> XUGCUGGCUAAGGGCCGAAAGX;> CUAUGCCUGCUG

The TNA backbone is composed of phosphodiester-linked 3′→2′ α-l-threofuranose sugars and, therefore, has one fewer atom in its repeating unit than RNA. Critically, TNA can form stable Watson−Crick duplexes with itself, DNA and RNA, such that the exchange of genetic information between these polymers appears feasible. Here, we examine the behaviour of TNA in nonenzymatic template-directed primer extension reactions from both a kinetic and a structural perspective. Taken together, we propose that structural constraints explain the diminished ability of TNA to engage in nonenzymatic template-directed primer extension, and we discuss the consequences of these observations for the plausibility of the involvement of TNA in the origin of primitive cells.

To gain insight into the structure of a reaction center containing a priming threo-nucleotide, we crystallized an RNA hairpin-monomer complex (TNA-P1), in which the RNA stem contained a 2′ terminal threo-guanosine (tG) residue followed by a single-nucleotide gap. One unactivated cytidine monophosphate (CMP) mononucleotide was sandwiched noncovalently between the tG primer and the downstream helper oligonucleotide, to mimic the bound monomer in the ground state prior to primer extension. We determined the structure to a resolution of 2.7 Å. The terminal tG residue at the 2′-end of the primer was well ordered, with the guanine nucleobase Watson–Crick base-paired with the templating cytidine. The threose sugar is in a C4′-exo conformation with the 2′ and 3′ hydroxyls pseudo-diaxial, consistent with a prior report from Egli et al. in which a TNA residue was present in the middle of an oligonucleotide. The 2′-OH group of the tG residue is oriented toward the phosphate of the incoming CMP monomer, which is Watson-Crick paired with the template. The distance between the P atom of the bound CMP and the 2′-OH of the tG primer is ∼3.2 Å, which appears favourable for attack, however as the monomer is unactivated CMP, the structure is not informative about the angle of attack with respect to the leaving group. Thus, a single threo-nucleotide at the end of an RNA duplex is accommodated with minimal structural perturbation. The largest deviations between the two structures are at the primer terminus, where the tG residue is shifted and twisted compared to the native RNA primer, with distances in the range of 1.5–2.4 Å between the corresponding atoms of the threose and ribose sugar rings. The tG residue has a glycosidic linkage torsion χ angle of –121°, compared to a typical χ angle of –168° for the ribonucleotides of the primer.N-[(1R,3R)-3-hydroxy-1-(hydroxymethyl)-3-phenylpropyl]pentadecanamide | C25 H43 N O3 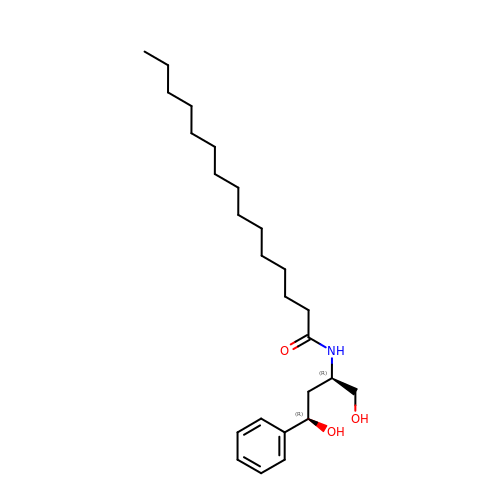| LFNPKXLKUQCCJV-DNQXCXABSA-N4-methyl-6-{[(3R,4R)-4-{[5-(pyridin-2-yl)pentyl]oxy}pyrrolidin-3-yl]methyl}pyridin-2-amine | C21 H30 N4 O | 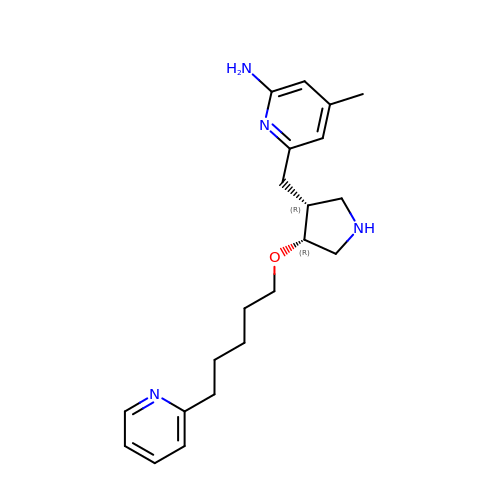CSFKTRORRCGDRY-XLIONFOSSA-N> MAAVILESIFLKRSQQKKKTSPLNFKKRLFLLTVHKLSYYEYDFERGRRGSKKGSIDVEKITCVETVIPEKNPPPERQIPRRGEESSEMEAASAAERFPYPFQVVYDEGPLYVFSPTEELRKRWIHQLKNVIRYNSDLVQKYHPCFWIDGQYLCCSQTAKNAMGCQILENRGGGSGGGGSGGGGSGGGGSGGGEIDPKDLTFLKELGTGQFGVVKYGKWRGQYDVAIRMIREGSMSEDEFIEEAKVMMNLSHEKLVQLYGVCTKQRPIFIITEYMANGCLLNYLREMRHRFQTQQLLEMCKDVCEAMEYLESKQFLHRDLAARNCLVNDQGVVKVSDFGMTRYVLDDEYTSSTGSKFPVKWASPEVLMYSKFSSKSDIWAFGVLMWEIYSLGKMPYERFTNSETAEHIAQGLRLPRPHLASERVYTIMYSCWHEKADERPSFKILLSNILDVMDEES

The TEC family kinase, BTK (Bruton’s tyrosine kinase) is best known as the target of ibrutinib (IMBRUVICA), the first-in-class covalent kinase active site inhibitor used to treat chronic lymphocytic leukemia, mantle cell lymphoma, Waldenström’s macroglobulinemia, and chronic graft-versus-host disease. The TEC and SRC kinases share the SH3–SH2–kinase domain arrangement (the ‘Src module’). In contrast, BTK contains an extended N-terminal region (PHTH–PRR) consisting of the phospholipid-binding Pleckstrin homology (PH) domain followed by a Tec homology (TH) domain and a long linker housing two proline-rich regions (PRR). Membrane-induced dimerization activates BTK and we present here a crystal structure of an activation loop swapped BTK kinase domain dimer that likely represents the conformational state leading to trans-autophosphorylation. Together, these data provide the first structural elucidation of full-length BTK and allow a deeper understanding of allosteric control over the BTK kinase domain during distinct stages of activation.

The first step in our redesign was to lengthen the linker between PHTH and kinase domain to reflect the flexibility and distance between the N- and C-terminal domains of BTK. We inserted GGSGG repeats that were either 22 or 32 amino acids in length. In addition, the new 1PHTH171-G(GGSGG)4/6G-396kinase659 constructs included PHTH β5–β6 loop mutations (Q91A, I92A, I94A, and I95A) to prevent formation of the ‘Saraste dimer‘ since that structure is associated with BTK activation. The structure of the PHTH–G(GGSGG)4G–kinase bound to GDC-0853 was determined to 2.1 Å. In the structure solved here (left), the longer linker between domains allows the PHTH domain to bind to the β-strands of the kinase domain N-lobe instead of the C-helix-binding site defined previously. Three PHTH domain side chains, R133, Y134, and R171, provide key interactions with the kinase domain in this new structure. The Y134 side chain inserts into the hydrophobic stack created by W421 and Y461 on the kinase domain N-lobe in a manner that mimics the L390 side chain position in the autoinhibited SH3–SH2–kinase structure. The guanidinium group of R171 participates in hydrogen bonds with the side chains of S453 and Q459 in the kinase domain. The guanidinium group of R133, in contrast, points back into the PHTH domain forming a hydrogen bond with the PHTH N130 side chain while the hydrophobic methylene groups of the R133 side chain contact I397 and Y461. The total solvent-excluded surface area of the PH–KD interface is 753.8 Å2.> NTPWQGYDINTNYYETIPQTNVVREYWFDIVNTTAALDGVERPVLLVNGQFPGPTIEANWGDTVKVHVTNRMENNGTAIHFHGIRQLYNNQMDGVAALTQCPVPPNSSYTYVWRAEEYGSSWYHSHFSLQAWEGVFGGILIHGPSTAEYDHDLGMVFLNDWSHQTVDEMYQSVLESQNPPHFQTGLINGSNIWVTADNQTVGRRFQTEFVPGQRYRLRLVNAAMHTHFRFSIDNHDLTVIASDFVPIVPFTTNNVPIGMGQRYDIIVTANQAPDNYWIRAIPQSFCSDNANSDNIKGVLHYEGAADNSDPTSTKWDYGDDIQCLDFSLDELVPWLALDADIGGAQMAESDVDFTPFGDVPLYLWTMGGNALNISWKDPTLQQTFEDPDKMDWKASQGVIEAAIPNKWTV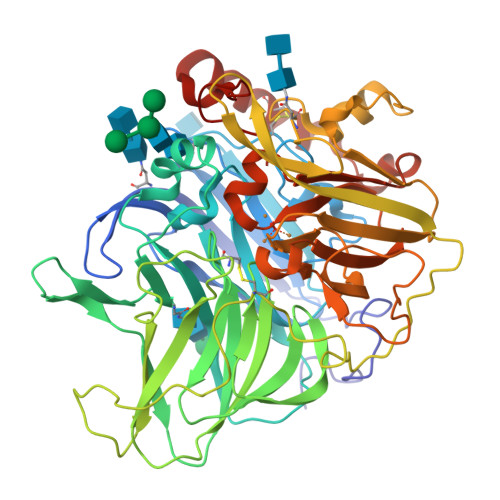LVVQTDLPVPHPIHLHGHDFYLLAQGFGQFNPQNVTLKTHNPPRRDTALMTAATPENGGGGYMVIGFPADNPGVWLIHCHIGFHATEGFAQQIVERQSEFNTFFSEDLLENTCDAWDEYAKVNPYGHQYRALAGPYESGI> GSMAE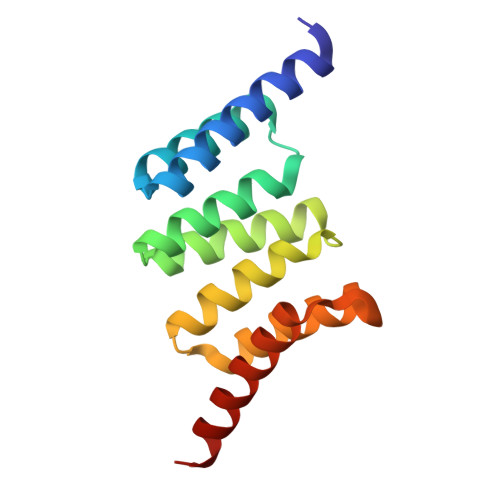TKAKAEDLKMQGNKAMANKDYELAINKYTEAIKVLPTNAIYYANRAAAHSSLKEYDQAVKDAESAISIDPSYFRGYSRLGFAKYAQGKPEEALEAYKKVLDIEGDNATEAMKRDYESAKKKVEQSLNL>TKKESFEDVLPSILNTITTNSELTEVPEVANWLKKVLEYNLAGGKKARGLTTLFAYEMLEKPENITEETIYLAKTLGWCVEILQGFLVMLDDIMDGSTTRRGVPCWYQLPEVGLAAVNDSSLMFSSIFYVLHAHFADKKIYTNLVELFNESLMHTSIGQHLDVTMERRQKSDYSLFTIERYNAIVKYKTAYYTYQLPVCLGMLLANISDPVLHQKAEDMCLEIGKFFQIQDDYIDCYGDESLTGKMGTDIQEAKCSWLAVMALQRCSASQKIVFTTCYGSKEPAHIERIKELYK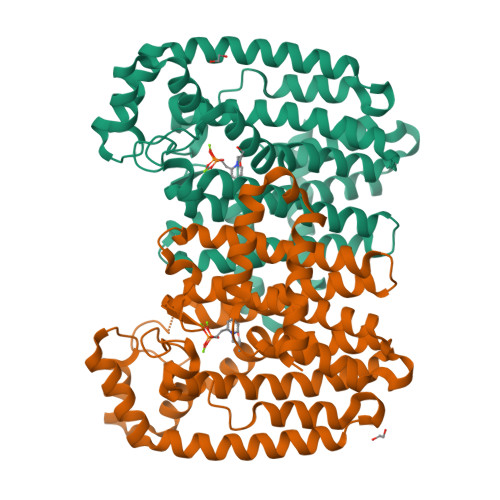QLQLPELYAQEETRMYESLIKQAHGLPSELSPALFVRLIHMIYKRNH[3x]>G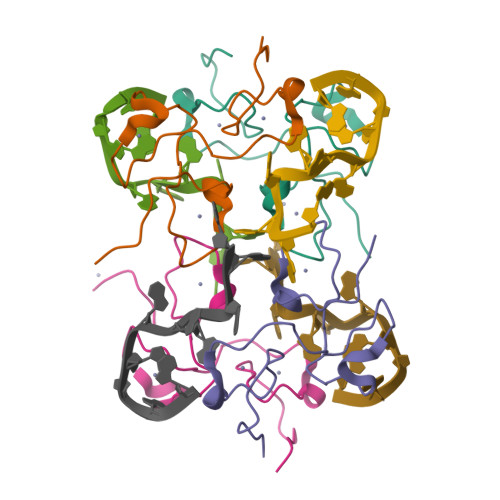SEKSLEQCKFGTHCTNKRCKYRHARSHIMCREGANCTRIDCLFGHPINEDCRFGVNCKNIYCLFRHPPGRVLPEKK[4x]7-HYDROXY-2-(4-HYDROXY-PHENYL)-CHROMAN-4-ONE 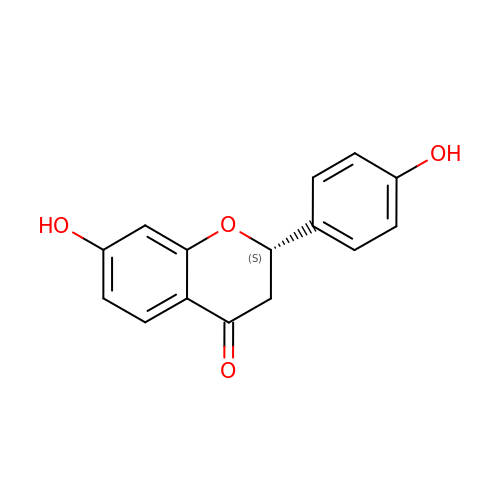| C15 H12 O4 | FURUXTVZLHCCNA-AWEZNQCLSA-N> SMQLNQYTLKDEIGKGSYGVVKLAYNENDNTYYA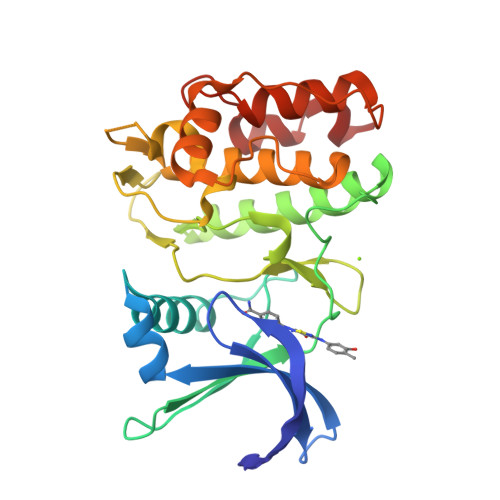MKVLSKKKLIRQAGFPRRPPPRGTRPAPGGCIQPRGPIEQVYQEIAILKKLDHPNVVKLVEVLDDPNEDHLYMVFELVNQGPVMEVPTLKPLSEDQARFYFQDLIKGIEYLHYQKIIHRDIKPSNLLVGEDGHIKIADFGVSNEFKGSDALLSNTVGTPAFMAPESLSETRKIFSGKALDVWAMGVTLYCFVFGQCPFMDERIMCLHSKIKSQALEFPDQPDIAEDLKDLITRMLDKNPESRIVVPEIKLHPWVTRH> GSMASEIHMTGPMCLIENTNGRLMANPEALKILSAITQPMVVVAIVGLYRTGKSYLMNKLAGKKKGFSLGSTVQSHTKGIWMWCVPHPKKPGHILVLLDTEGLGDVEKGDNQNDSWIFALAVLLSSTFVYNSIGTINQQAMDQLYYVTELTHRIRSKSSPDENENEVEDSADFVSFFPDFVWTLRDFSLDLEADGQPLTPDEYLTYSLKLKKGTSQKDETFNLPRLCIRKFFPKKKCFVFDRPVHRRKLAQLEKLQDEELDPEF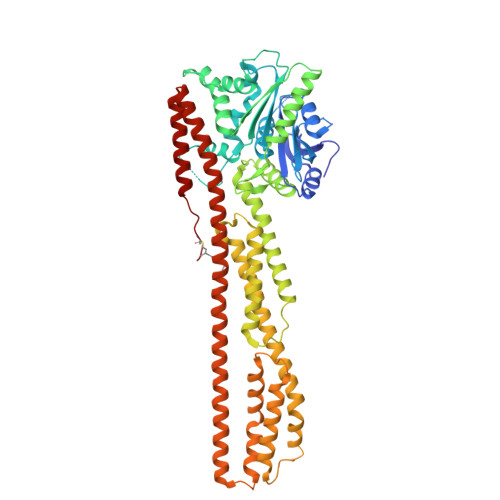VQQVADFCSYIFSNSKTKTLSGGIQVNGPRLESLVLTYVNAISSGDLPCMENAVLALAQIENSAAVQKAIAHYEQQMGQKVQLPTETLQELLDLHRDSEREAIEVFIRSSFKDVDHLFQKELAAQLEKKRDDFCKQNQEASSDRCSALLQVIFSPLEEEVKAGIYSKPGGYRLFVQKLQDLKKKYYEEPRKGIQAEEILQTYLKSKESMTDAILQTDQTLTEKEKEIEVERVKAESAQASAKMLQEMQRKNEQMMEQKERSYQEHLKQLTEKMENDRVQLLKEQERTLALKLQEQEQLLKEGFQKESRIMKNEIQDLQTKMRRRKACTIS>MMSETAPLPSASSALEDKAASAPVVGIIMGSQSDWETMRHADALLTELEIPHETLIVSAHRTPDRLADYARTAAERGLNVIIAGAGGAAHLPGMCAAWTRLPVLGVPVESRALKGMDSLLSIVQMPGGVPVGTLAIGASGAKNAALLAASILALF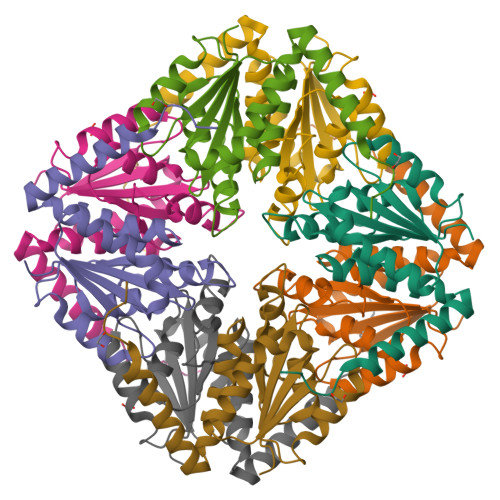NPALAARLETWRALQTASVPNSPITEDK[2x]ethyl 5-[1,3-benzodioxol-5-ylmethyl(ethyl)carbamoyl]-2,4-dimethyl-1~{H}-pyrrole-3-carboxylate 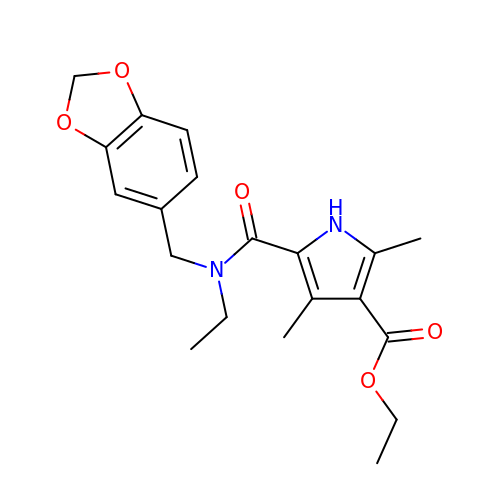| C20 H24 N2 O5 | MTVMTCROAUSHKU-UHFFFAOYSA-N>[2x]VTSSPFKTIKSDEIFAAAQKLMPGGVSSPVRAFKSVGGQPIVFDRVKDAYAWDVDGNRYIDYVGTWGPAICGHAHPEVIEALKVAMEKGTSFGAPCALENVLAEMVNDAVPSIE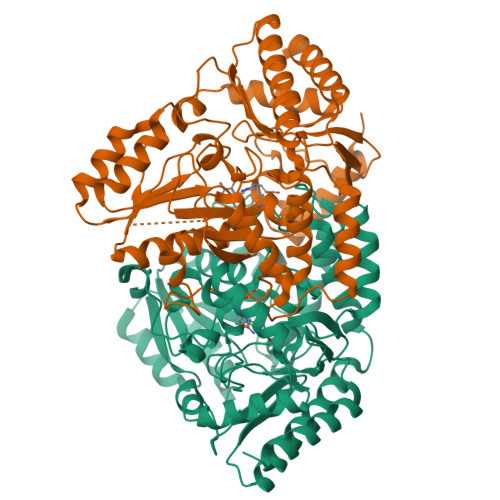MVRFVNSGTEACMAVLRIMRAYTGRDKIIKFEGCYHGHADMFLVKAGSGVATLGLPSSPGVPKKTTANTLTTPYNDLEAVKALFAENPGEIAGVILEPIVGNSGFIVPDAGFLEGLREITLEHDALLVFDEVMTGFRIAYGGVQEKFGVTPDLTTLGKIIGGGLPVGAYGGKREIMQLVAPAGPMYQAGTLSGNPLAMTAGIKTLELLRQPGTYEYLDQITKRLSDGLLAIAQETGHAACGGQVSGMFGFFFTEGPVHNYEDAKKSDLQKFSRFHRGMLEQGIYLAPSQFEAGFTSLAHTEEDIDATLAAARTVMSAL>[4x]QDAKAGEAVFKQCMT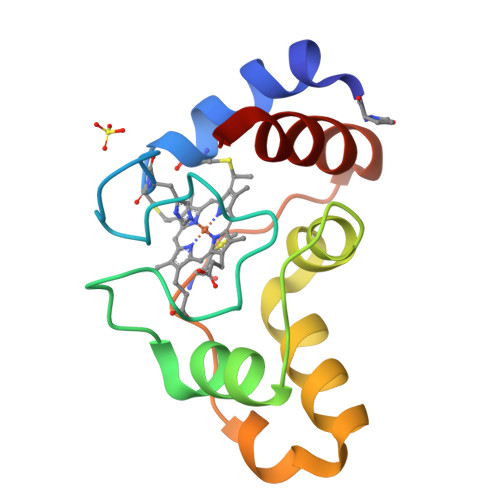CHRADKNMVGPALAGVVGRKAGTAAGFTYSPLNHNSGEAGLVWTADNIVPYLADPNAFLKKFLTEKGKADQAVGVTKMTFKLANEQQRKDVVAYLATLK>MVMIDLYTAATPNGHKVSIALEEMGLPYRVHALSFDKKEQKAPEFLRINPNGRIPAIVDRDNDDFAVFESGAILIYLAEKTGQLMPADVKGRSRVIQWLMFQMGGVGPMQGQANVFFRYFPEKLQGAIDRYQHETRRLYEVLDGRLGEAEYLAGDYSIADIATYPWVRIHDWSGVAVDGLDNLQRWIAAIEARPAVQRGLLVPRREKEGDDAIRT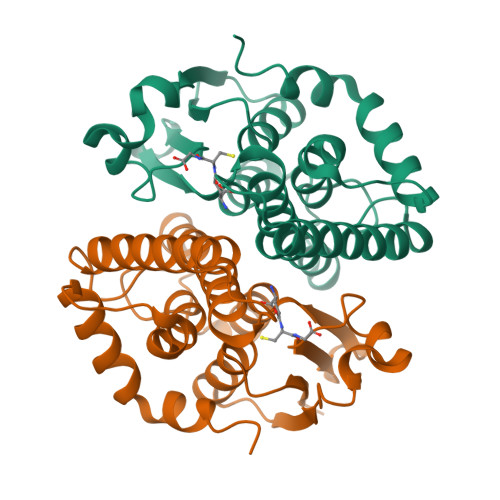AQSMLTRAENLYFQSHHHHHHWSHPQFEK[2x]> GSHMDELYRQSLEII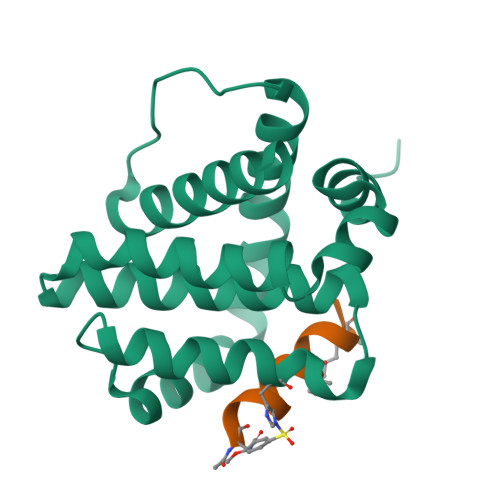SRYLREQATGAKDTKPMGRSGATSRKALETLRRVGDGVQRNHETAFQGMLRKLDIKNEDDVKSLSRVMIHVFSDGVTNWGRIVTLISFGAFVAKHLKTINQESCIEPLAESITDVLVRTKRDWLVKQRGWDGFVEFFHVED;> XAIAEQLRAIGDAFX METHYL 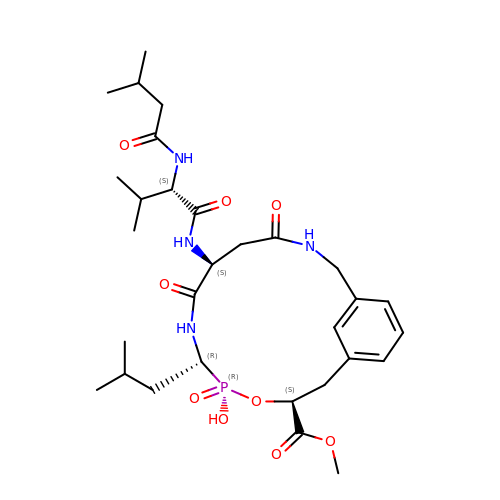CYCLO[(2S)-2-[[(1R)-1-(N-(L-N-(3-METHYLBUTANOYL)VALYL-L-ASPARTYL)AMINO)-3-METHYLBUTYL]HYDROXYPHOSPHINYLOXY]-3-(3-AMINOMETHYL)PHENYLPROPANOATE | C30 H47 N4 O9 P | BOYAGOIPWLIWCX-IDJLGEMNSA-N>HMKNVLLIGARGALGRAVANAFANGKWSIISVDQAAAVQQGDECCAVNPASSIEELQQAYKSAVTGLKVDAVINVAGGWAGGSVADASTAASTELMLRQSLFSSVAAAHVFSTQGEKNGLLLLTGAAAA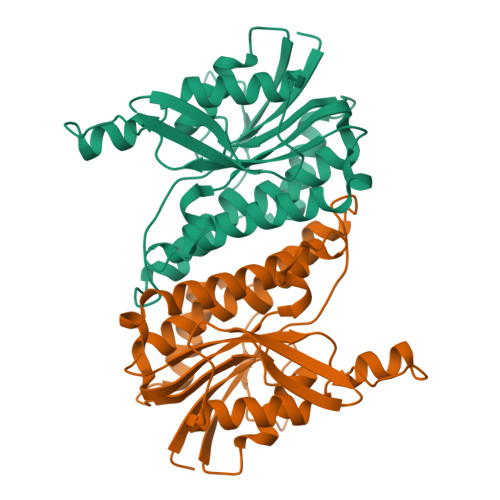VSPTPGMIGYGTAKSAVHFLCQSIAEDPSVLPTDASVLAILPTILDTPGNRSAMPHADRSTWTSLEDVAQQIVEWSNGSRRPASGSLVKIVTENSKTRFIV[3x]>MNQSVSSLAEKDIQYQLHPYTNARLHQELGPLIIERGQGIYVYDDQGKGYIEAMAGLMSVALGFSNQRLIKAAEQQFNTLPFYHLLNHKSHRPSIELAEKLIEMAPVPMSKVFFTNSGSEANDTVVKFVWYLNNALGKPAKKKFISRVNGYHGVTVASASLTGLPGNQRGFDLPLPGFLHVGCPHHYRFALAGESEEHFADRLAVELEQKILAEGPETIAAFIGEPLMGAGGVIVPPRTYWEKIQKVCRKYDILVIADEVICGFGRTGQMFGSQTFGIQPDIMVLSKQLSSSYQPIAAILINAPVFEGIADQSQALGALGHGFTGSGHPVATAVALENLKIIEEESLVEHAA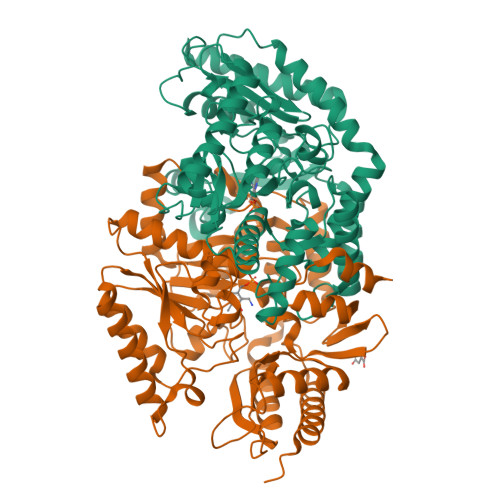QMGQLLRSGLQHFIDHPLVGEIRGCGLIAAVELVGDRVSKAPYQALGTLGRYMAGRAQEHGMITLAMGDAVAFCPPLIVNEQEVGMIVERFARALDDTTQWVGPGGHHHHHH[2x]>GDSLSIHQLAAQGELDQLKEHLRKGDNLVNK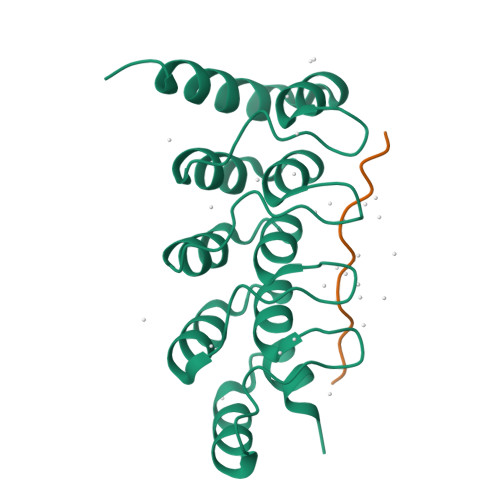PDERGFTPLIWASAFGEIETVRFLLEWGADPHILAKERESALSLASTGGYTDIVGLLLERDVDINIYDWNGGTPLLYAVRGNHVKCVEALLARGADLTTEADSGYTPMDLAVALGYRKVQQVIENHILKLFQSNLVPADPE[2x];>[2x]KAFVHMPTLPNLDFHKT> MKKHHHHHHGSLVPRGSKLEINKFNYNDPIDGINVITMRPPRHSDKINKGKGPFKAFQVIKNIWIVPERYNFTNNTNDLNIPSEPIMEADAIYNPNYLNTPSEKDEFLQGVIK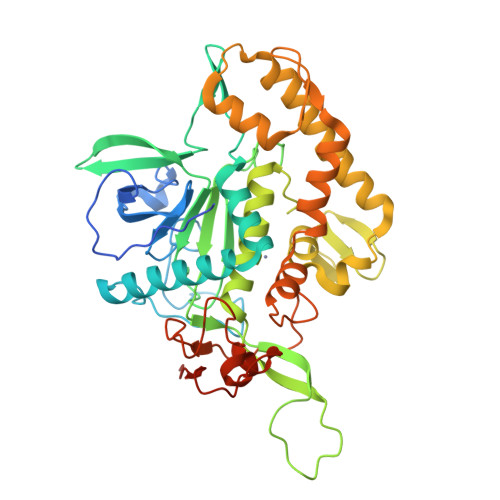VLERIKSKPEGEKLLELISSSIPLPLVSNGALTLSDNETIAYQENNNIVSNLQANLVIYGPGPDIANNATYGLYSTPISNGEGTLSEVSFSPFYLKPFDESYGNYRSLVNIVNKFVKREFAPDPASTLMHELVHVTHNLYGISNRNFYYNFDTGKIETSRQQNSLIFEELLTFGGIDSKAISSLIIKKIIETAKNNYTTLISERLNTVTVENDLLKYIKNKIPVQGRLGNFKLDTAEFEKKLNTILFVLNESNLAQRFSILVRKHYLKERPIDPIYVNILDDNSYSTLEGFNISSQGSNDFQGQLLESSYFEKIESNALRAFIKICPRNG> GPLGSMNEMENTDPVLQDDLVSKYERELSTEQEEDTPVILTQLNEDGTTSNYFDKRKLKIAPRSTLQFKVGPPFELVRDYCPVVESHTGRTLDLRIIPRIDRGFDHIDEEWVGYKRNYFTLVSTFETANCDLDTFLKSSFDLLVEDSSVEGRLRVQYFAIKIKAKNDDDDTEINLVQHTAKRDKGPQFCPSVCPLVPSPL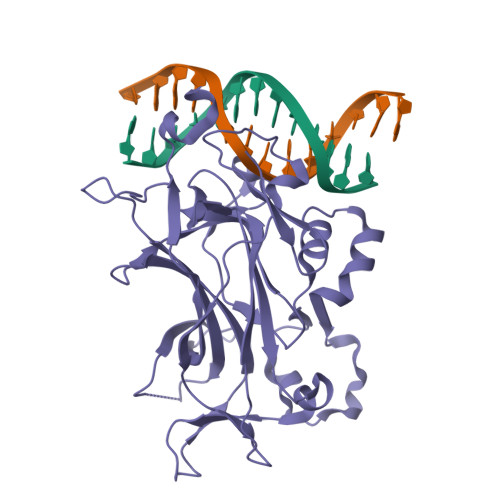PKHQTIREASNVRNITKMKKYDSTFYLHRDHVNYEEYGVDSLLFSYPEDSIQKVARYERVQFASSISVKKPSQQNKHFSLHVILGAVVDPDTFHGENPGIPYDELALKNGSKGMFVYLQEMKTPPLIIRGRSPSNYASSQRITVR>[420x]MARQNSAAKTTAKSKTDPATEKPKDDTLPDSTDDASPTAPETPATKPDSASDEVEGVFVRATVERRCRAGFCFDKEGQGFADGVLSDEQLEALESDPLLKVERCTFSGNQEGE;>[415x]MAIITPALISALKTSFQKHFQDALATAPSTYLQVATVIPSTTASNTYGWLGQFPKLREWIGQRVIKDMAAQGYQITNKLFESTVGVKRTDIEDDNLGVYGPLMQEMGRAAGAHPDELVFALLKAGNANLCYDGQNFFDTDHPVYPNVDGTGTATTVSNLFAPAADPGAAWYLLDTSRSLKPLIYQERMKPSFTSMTKEDDEQVFMADEYRYGVRSRCNVGFGFWQLAAMSTEELNQVNFEKVYDAMRNQKADGGRPLDIRPNLLVVPTTLRSKAKEVVGVQRLANGADNPNFELVQVLDTAWLN;>[12x]MSYCTLADLIEQYSEQKIRE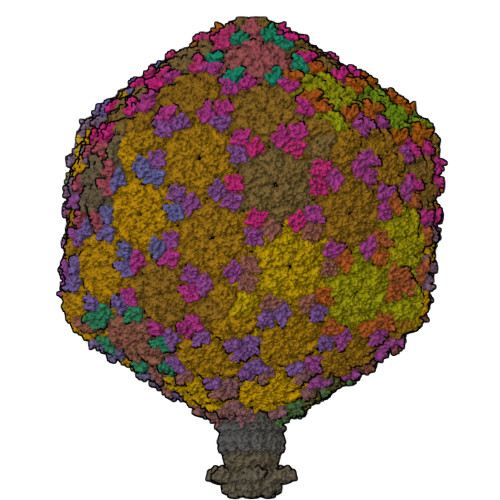VSDRVNKPATTIDTVIVDRAIADADSEIDLHLHGRYQLPLASVPTALKRIACGLAYANLHIVLKEENPVYKTAEHLRKLLSGIANGKLSLALDADGKPAPVANTVQISEGRNDWGADW;>MAQIVDVYGNPIRTQQLREPQTSRLAGLAKEFAQHPAKGLTPAKLARILVEAEQGNLQAQAELFMDMEERDAHLFAEMSKRKRAILGLDWAVEPPRNASAAEKADADYLHELLLDLEGLEDLLLDALDGIGHGYSCIELEWALQGREWMPLAFHHRPQSWFQLNPEDQNELRLRDNSPAGEALQPFGWIIHRPRARSGYVARSGLFRVLAWPYLFRHYATSDLAEMLEIYGLPIRLGKYPPGTADEEKATLLRAVTGLGHAAAGIIPETMAIDFQQAAQGSSDPFLAMMRQSEDAISKAVLGGTLTSTTSQSGGGAFALGQVHNEVRHDLLASDARQLAATLSRDLLWPLLVLNRPGSPDVRRAPRLVFDLREQADITSMAQSIPALVNVGLEIPSAWVYDKLGIPQPAKNEPVLRSAAQPAILSRQHGQRVAALATIVGPRYGDQQALDKALASLPAKDMQDQVNDLLAPLLEAVNRGDSETELLGALAEAFPDMDDSALTDALHRLLFAADTWGRLHGNLDRID[12x];>MSDPFDYLFLEPLLIERIRSEVPGLAIVSGVPDLATLSEQDQPAPSAYVVYLGDETGTGADHQGGQRAIQTVGQQWAVVLVVHYADSSNSGEGARREAGPLLGRLVKALTGWAPAIDVAPLARSARQSPATYASGYLYFPLVFTARFVYPRIKSWKP[6x];>MAQETYFYGQGEIDAAPIVNGVLGKWRWIQDVSAMSIQLAVEKVEHKESYSGQKALVRSFPIGKTATVNITLHSIGPDNLALTLYGKVVAKAAGSVTGEVLPADLVAGDVIRLANFGVSELVITDSASSPAPLDPQYYALRADGAYGEVQLLGLPTPAPTQPFKAAYEYAATKQVGMFTAPQPTVALRYKGINLAEGGAPVIVELYKVATDPLQELALISDGNTVAGMQISGGILLDTSKPDTGDLGRFGRIIQLG[6x]>MTERIRNVALRSKVCPAETASELIKHGDVVGTSGFTGAGYPKEVPKALAQRMEAAHDRGEKYQISLITGASTGPQLDGELAKANGVYFRSPFNTDATMRNRINAGETEYFDNHLGQVAGRAVQGNYGKFNIALVEATAITED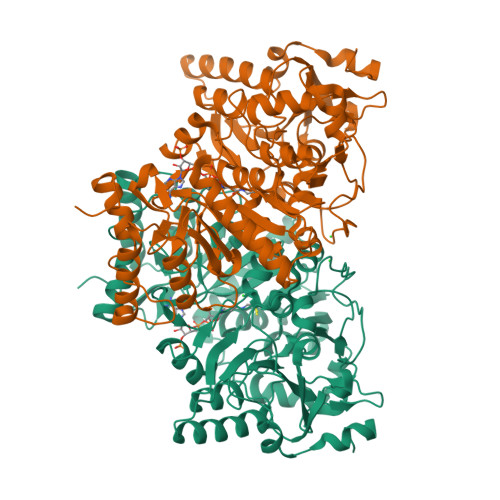GGIVPTSSVGNSQTFLNLAEKVIIEVNEWQNPMLEGIHDIWDGNVSGVPTRDIVPIVRADQRVGGPVLRVNPDKIAAIVRTNDRDRNAPFAAPDETAKAIAGYLLDFFGHEVKQNRLPPSLLPLQSGVGNVANAVLEGLKEGPFENLVGYSAVIQDGMLAMLDSGRMRIASASSFSLSPEAAEEINNRMDFFRSKIILRQQDVSNSPGIIRRLGCIAMNGMIEADIYGNVNSTRVMGSKMMNGIGGSGDFARSSYLSIFLSPSTAKGGKISAIVPMAAHVDHIMQDAQIFVTEQGLADLRGLSPVQRAREIISKCAHPDYRPMLQDYFDRALKNSFGKHTPHLLTEALSWHQRFIDTGTMLPSSLEHHHHHH[2x]>MTDVNASSESRLAALEARVTELEDLNAIRRLQWAYGYYIDYNRPEEVAGLFAKDGAVVFLSGEYVGYEGVMRLYGTWFQNLFTGGRRGPVHGLLLDQFQLQDVITIAPDGQTAKGRFRGILAGGWHDDIVKDKPEGMPQQFWESGIYENDYVKEDGVWKIKRLDYMMQWQADYETG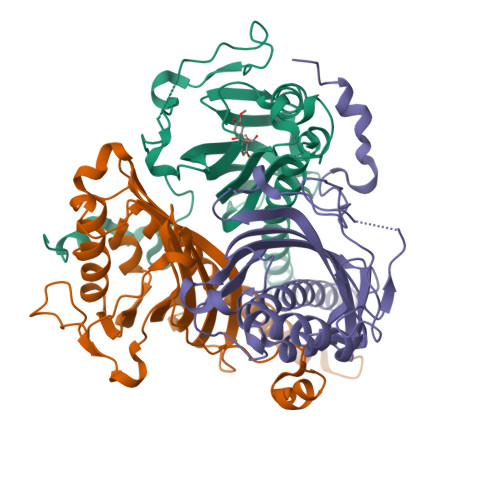WSKTIAHLQPAAVCFPENPIGPDRLLPETEVRQTWPHRAEVPMSFAHPVLAKAFAVGEFTKLQKKWPLEHHHHHH[3x]>KDKEFQVLFVLTILTLISGTIFYSTVEGLRPIDALYFSVVTLTTVGYGDFSPQTDFGKIFTILYIFIGIGLVFGFIHKLAVNVQLPSIL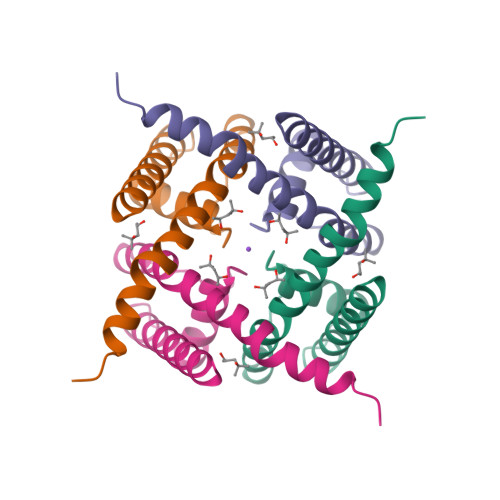SNLVPR[2x]> MSKKPVALIILDGFALRDETYGNAVAQANKPNFDRYWNEYPHTTLKACGE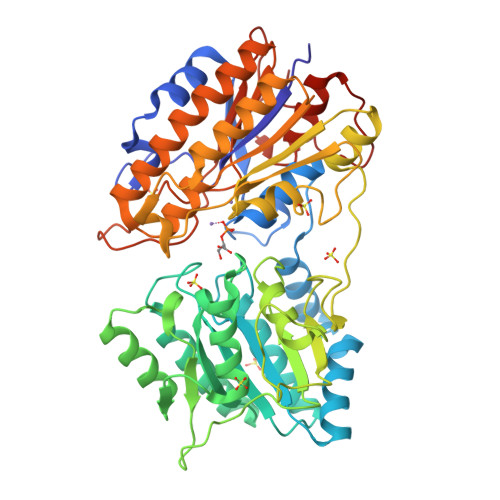AVGLPEGQMGNSEVGHLNIGAGRIVYQSLTRINIAIREGEFDRNETFLAAMNHVKQHGTSLHLFGLLSDGGVHSHIHHLYALLRLAAKEGVKRVYIHGFLDGRDVGPQTAPQYIKELQEKIKEYGVGEIATLSGRYYSMDRDKRWDRVEKAYRAMVYGEGPTYRDPLECIEDSYKHGIYDEFVLPSVIVREDGRPVATIQDNDAIIFYNFRPDRAIQISNTFTNEDFREFDRGPKHPKHLFFVCLTHFSETVAGYVAFKPTNLDNTIGEVLSQHGLRQLRIAETEKYPHVTFFMSGGREEEFPGEDRILINSPKVPTYDLKPEMSAYEVTDALLKEIEADKYDAIILNYANPDMVGHSGKLEPTIKAVEAVDECLGKVVDAILAKGGIAIITADHGNADEVLTPDGKPQTAHTTNPVPVIVTKKGIKLRDGGILGDLAPTMLDLLGLPQPKEMTGKSLIVK> GGGGUGUGCCCGGCAUGGGUGCAGUCUAUAGGGUGAGAGUCCCGAACUG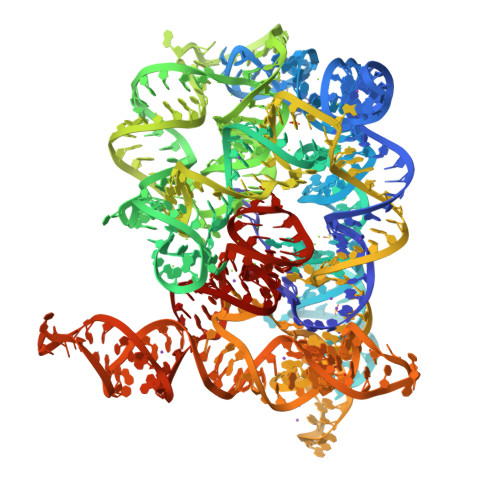UGAAGGCAGAAGUAACAGUUAGCCUAACGCAAGGGUGUCCGUGGCGACAUGGAAUCUGAAGGAAGCGGACGGCAAACCUUCGGUCUGAGGAACACGAACUUCAUAUGAGGCUAGGUAUCAAUGGAUGAGUUUGCAUAACAAAACAAAGUCCUUUCUGCCAAAGUUGGUACAGAGUAAAUGAAGCAGAUUGAUGAAGGGAAAGACUGCAUUCUUACCCGGGGAGGUCUGGAAACAGAAGUCAGCAGAAGUCAUAGUACCCUGUUCGCAGGGGAAGGACGGAACAAGUAUGGCGUUCGCGCCUAAGCUUGAACCGCCGUAUACCGAACGGUAGGUACGGUGGUGUG> MRLSYEALEWRTPIENSTEPVSLPPPPPFFGQERAREALELAIRGGFHAYLVGPPSLGKHEALLAYLSTQSVETPPDLLYVPLSERKVAVLTLPSGQEIHLAEAVEGLLLEVNRLDELFRQGSFLREKTQLEARFKEAREQQLEALRREAQEAGFALSTNGERLELTGPGPVPAELSARLEEVTLGSLAASAELEVALRRLRRDWALHYLNNRFEPLFQRFPQARAYLEALRARLARYAETGEPLDPAQWRPNLLTSSSSGTPPPIVYEPYATAPRLFGRLDYLVDRGVWSTNVSLIRPGAVHRAQGGYLILDALSLKREGTWEAFKRALRNGQVEPVTEPQAPAGLEVEPFPIQMQVILVGTPEAFEGLEEDPAFSELFRIRAEFSPTLPASPENCTALGGWLLAQGFQLTQGGLTRLYDEARRMAEQRDRMDARLVEIRALAEEAAVLGGGLLTAE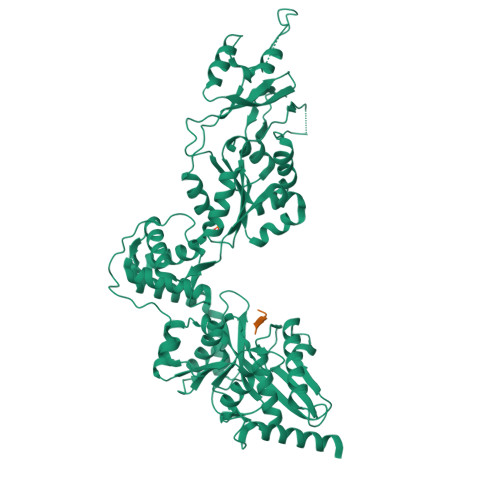SVEQAIAAREHRSFLSEEEFLRAVQEGVIRLRTTGRAVGEVNSLVVVEAAPYWGRPARLTARAAPGRDHLISIDREAGLGGQIFHKAVLTLAGYLRSRYIEHGSLPVTISLAFEQNYVSIEGASAGLAELVAALSAIGNLPLRQDLAVTGAVDQTGKVLAVGAINAKVEGFFRVCKALGLSGTQGVILPEANLANLTLRAEVLEAVRAGQFHIYAVETAEQALEILAGARMEGFRGLQEKIRAGLEAFARLEEGHDKEDREKLAAALEHHHHHH;> APEAV(2~{R},3~{R},5~{R})-3-acetamido-5-fluoranyl-2-[(1~{R},2~{R})-1,2,3-tris(oxidanyl)propyl]-2,3,4,5-tetrahydropyran-1-ium-6-carboxylic 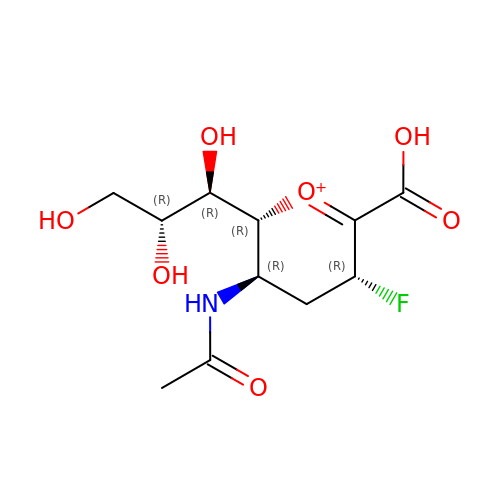acid | C11 H17 F N O7 | JMALISIZGRCKCG-VRRGKTLJSA-O>MEPGRGG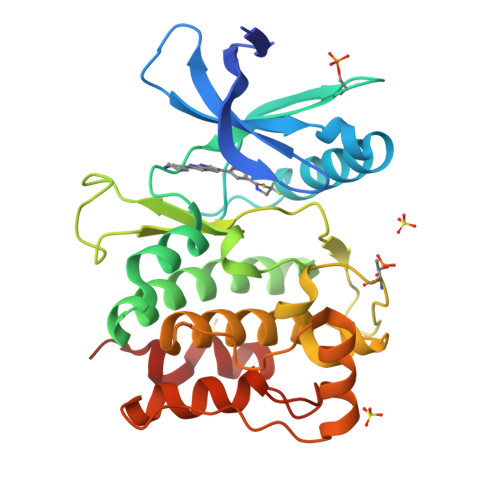TETVGKFEFSRKDLIGHGAFAVVFKGRHRAAHDLEVAVKCINKKNLAKSQTLLGKEIKILKELKHENIVALYDFQEMANSVYLVMEYCNGGDLADYLHAMRTLSEDTIRLFLQQIAGAMRLLHSKGIIHRDLKPQNILLSNPAGRRANPNSIRVKIADFGFARYLQSNMMAATLCGSPMYMAPEVIMSQHYDGKADLWSIGTIVYQCLTGKAPFQASSPQDLRLFYEKNKTLVPTIPRETSAPLRQLLLALLQRNHKDRMDFDEFFHHPFLDASPS[2x]>[8x]MMVISEKVRKALNDQLNREIYSSYLYLSMATYFDAEGFKGFAHWMKKQAQEELTHAMKFYEYIYERGGRVELEAIEKPPSNWNGIKDAFEAALKHEEFVTQSIYNILELASEEKDHATVSFLKWFVDEQVEEEDQVREILDLLEKANGQMSVIFQLDRYLGQRE

Four helix bundles are also attractive for synthetic chemists because its interfaces are dominated by side chain and side chain interactions, which can be more tunable than β-strands. This study focuses on TmFtn, a naturally dimeric protein consisting of two antiparallel four helix bundles, as shown in Supplementary Fig. 1. Thermotoga maritima ferritin (TmFtn) naturally occurs as a dimer; twelve of these dimers interact with each other in a head-to-side manner to generate 24-meric hollow protein nanocage in the presence of Ca2+ or PEG. By tuning two contiguous dimeric proteins to interact in a fully or partially side-by-side fashion through protein interface redesign, we can render the self-assembly transformation of such dimeric building blocks from the protein nanocage to filament, nanorod and nanoribbon in response to multiple external stimuli.

Consistent with these recent findings, our results show that, in solution, purified TmFtn molecules exist as dimers and can self-assemble into 24-meric hollow protein nanocage in the presence of Ca2+, and addition of EDTA causes the formed protein nanocage disassembly back into its dimeric form, indicative of a reversible process of protein assembly. The crystal structure of 24-meric Tmftn determined at a resolution of 2.2 Å shows that one calcium ion located nearby C3–C4 interface is coordinated with two acidic residues (Glu51 and Glu132) and three water molecules. Careful analyses of the crystal structure revealed that a group of acidic amino acid residues are lined along with the C3–C4 interface, producing electrostatic repulsion along with this interface in the absence of calcium ions. This might be an important reason why TmFtn molecules naturally exist as protein dimers in solution in the absence of metal ions. In contrast, calcium ions near the C3–C4 interface can essentially eliminate such electrostatic repulsion through their interaction with the acidic residues, strengthening the stability of C3–C4 interface, finally producing the 24-meric protein nanocage. Besides, each protein nanocage is composed of 12 protein dimers, and any of the 2 adjacent protein dimers interact with each other in a head-to-side manner. Based on these findings, it is reasonable to believe that calcium ions facilitate the interaction of these protein dimers in a head-to-side manner, resulting in the formation of hollow protein nanocage. In contrast, native TmFtn exhibits a different packing pattern in its crystal where 12 TmFtn dimers assemble into a 24-mer protein cage.>[2x]MSEFNITETYLRFLEEDTEMTMPIAAIEALVTLLRIKTPETAAEMINTIKSSTEELIKSIPNSVSLRAGCDIFMRFVLRNLHLYGDWENCKQHLIENGQLFVSRAKKSRNKIAEIGVDFIADDDIILVHGYSRAVFSLLNHAANKFIRFRCVVTESRPSKQGNQLYTLLEQKGIPVTLIVDSAVGAVIDKVDKVFVGAEGVAESGGIINLVGTYSVGVLAHNARKPFYVVTESHKFVRMFPLSSDDLPMAGPPLDFTRRTDDLEDALRGPTIDYTAQEYITALITDLGVLTPSAVSEELIKMWYD;>[2x]MSESEAKSRSATPPSKAKQATPTTTAAANGEKKLTNKELKELKKQEKAAKRAAMKQANGISIEQQQQQAQMKKEKKQLQREQQQKREQKQKNANKKKQNERNVKKSTLFGHLETTEERRATILALTSAVSSPKTSRITAAGLMVPVVASALSGSNVLTASSLMPVGPNASSTVSASAPASTTTTLPASSAALSAGTSSASTNTPTAIQQEIASSNASDVAKTLASISLEAGEFNVIPGISSVIPTVLEQSFDNSSLISSVKELLLNKDLIHPSILLLTSHLAHYKIVGSIPRCIAMLEVFQIVIKDYQTPKGTTLSRNLTSYLSHQIDLLKKARPLSVTMGNAIRWLKQEISLIDPSTPDKAAKKDLCEKIGQFAKEKIELADQLIIDNASTQIEESTTIVTYGSSKVLTELLLHNAISLKKNIKVIVVDSRPLFEGRKMAETLRNAGVNVMYALITSLDTIFNMDVDYVFLGAHSILSNGFLYSRAGTAMLAMSAKRRNIPVLVCCESLKFSQRVQLDSVTFNELADPNDLVNIDYENPVERRGNKGALLNQFIKERKFEKKKLAMENKPKGNKIGGKKGSEGESKDASNEEDSNSKNILDGWQELPSLNIVNILYDLTPPEYIKKVITEFGALPPSSVPVILREYKGSA;>MSSQAFTSVHPNAATSDVNVTIDTFVAKLKRRQVQGSYAIALETLQLLMRFISAARWNHVNDLIEQIRDLGNSLEKAHPTAFSCGNVIRRILAVLRDEVEEDTMSTTVTSTSVAEPLISSMFNLLQKPEQPHQNRKNSSGSSSMKTKTDYRQVAIQGIKDLIDEIKNIDEGIQQIAIDLIHDHEILLTPTPDSKTVLKFLITARERSNRTFTVLVTEGFPNNTKNAHEFAKKLAQHNIETLVVPDSAVFALMSRVGKVIIGTKAVFVNGGTISSNSGVSSVCECAREFRTPVFAVAGLYKLSPLYPFDVEKFVEFGGSQRILPRMDPRKRLDTVNQITDYVPPENIDIYITNVGGFNPSFIYRIAWDNYKQIDVHLDKNKA[2x];>MAGKKGQKKSGLGNHGKNSDMDVEDRLQAVVLTDSYETRFMPLTAVKPRCLLPLANVPLIEYTLEFLAKAGVHEVFLICSSHANQINDYIENSKWNLPWSPFKITTIMSPEARCTGDVMRDLDNRGIITGDFILVSGDVLTNIDFSKMLEFHKKMHLQDKDHISTMCLSKASTYPKTRTIEPAAFVLDKSTSRCIYYQDLPLPSSREKTSIQIDPELLDNVDEFVIRNDLIDCRIDICTSHVPLIFQENFDYQSLRTDFVKGVISSDILGKHIYAYLTDEYAVRVESWQTYDTISQDFLGRWCYPLVLDSNIQDDQTYSYESRHIYKEKDVVLAQSCKIGKCTAIGSGTKIGEGTKIENSVIGRNCQIGENIRIKNSFIWDDCIIGNNSIIDHSLIASNATLGSNVRLNDGCIIGFNVKIDDNMDLDRNTKISASPLKNAGSRMYDNESNEQFDQDLDDQTLAVSIVGDKGVGYIYESEVSDDEDSSTEACKEINTLSNQLDELYLSDDSISSATKKTKKRRTMSVNSIYTDREEIDSEFEDEDFEKEGIATVERAMENNHDLDTALLELNTLRMSMNVTYHEVRIATITALLRRVYHFIATQTLGPKDAVVKVFNQWGLLFKRQAFDEEEYIDLMNIIMEKIVEQSFDKPDLILFSALVSLYDNDIIEEDVIYKWWDNVSTDPRYDEVKKLTVKWVEWLQNADEESSSEEE[2x];>[2x]MSIQAFVFCGKGSNLAPFTQPDFPFQTQNKDSTAATSGDKLNELVNSALDSTVINEFMQHSTRLPKALLPIGNRPMIEYVLDWCDQADFKEISVVAPVDEIELIESGLTSFLSLRKQQFELIYKALSNSNHSHHLQDPKKINFIPSKANSTGESLQKELLPRINGDFVILPCDFVTDIPPQVLVDQFRNRDDNNLAMTIYYKNSLDSSIDKKQQQKQKQQQFFTVYSENEDSERQPILLDVYSQRDVTKTKYLQIRSHLLWNYPNLTVSTKLLNSFIYFCSFELCQLLKLGPQSMSRQASFKDPFTGNQQQQNPPTTDDDEDRNHDDDDDYKPSATSIQPTYFKKKNDLILDPINCNKSLSKVFRDLSRRSWQHSKPREPIGIFILPNETLFIRANNLNAYMDANRFVLKIKSQTMFTKNIQIQSAAIGADAIVDPKCQISAHSNVKMSVLGTQANIGSRCRVAGSLLFPGVHLGDEVILENCIIGPMAKIGSKCKLSNCYIEGHYVVEPKNNFKGETLANVYLDEDEEDELIYDDSVIAGESEIAEETDSDDRSDEDSDDSEYTDEYEYEDDGLFER;>[2x]MSTSHCRFYENKYPEIDDIVMVNVQQIAEMGAYVKLLEYDNIEGMILLSELSRRRIRSIQKLIRVGKNDVAVVLRVDKEKGYIDLSKRRVSSEDIIKCEEKYQKSKTVHSILRYCAEKFQIPLEELYKTIAWPLSRKFGHAYEAFKLSIIDETVWEGIEPPSKDVLDELKNYISKRLTPQAVKIRADVEVSCFSYEGIDAIKDALKSAEDMSTEQMQVKVKLVAAPLYVLTTQALDKQKGIEQLESAIEKITEVITKYGGVCNITMPPKAVTATEDAELQALLESKELDNRSDSEDDEDESDDE;>MSSDLAAELGFDPALKKKKKTKKVIPDDFDAAVNGKENGSGDDLFAGLKKKKKKSKSVSADAEAEKEPTDDIAEALGELSLKKKKKKTKDSSVDAFEKELAKAGLDNVDAESKEGTPSANSSIQQEVGLPYSELLSRFFNILRTNNPELAGDRSGPKFRIPPPVCLRDGKKTIFSNIQDIAEKLHRSPEHLIQYLFAELGTSGSVDGQKRLVIKGKFQSKQMENVLRRYILEYVTCKTCKSINTELKREQSNRLFFMVCKSCGSTRSVSSIKTGFQATVGKRRRM[2x];>[2x]MSDLQDQEPSIIINGNLEPVGEPDIVEETEVVAQETQETQDADKPKKKVAFTGLEEDGETEEEKRKREFEEGGGLPEQPLNPDFSKLNPLSAEIINRQATINIGTIGHVAHGKSTVVRAISGVQTVRFKDELERNITIKLGYANAKIYKCQEPTCPEPDCYRSFKSDKEISPKCQRPGCPGRYKLVRHVSFVDCPGHDILMSTMLSGAAVMDAALLLIAGNESCPQPQTSEHLAAIEIMKLKHVIILQNKVDLMREESALEHQKSILKFIRGTIADGAPIVPISAQLKYNIDAVNEFIVKTIPVPPRDFMISPRLIVIRSFDVNKPGAEIEDLKGGVAGGSILNGVFKLGDEIEIRPGIVTKDDKGKIQCKPIFSNIVSLFAEQNDLKFAVPGGLIGVGTKVDPTLCRADRLVGQVVGAKGHLPNIYTDIEINYFLLRRLLGVKTDGQKQAKVRKLEPNEVLMVNIGSTATGARVVAVKADMARLQLTSPACTEINEKIALSRRIEKHWRLIGWATIKKGTTLEPIA

Eukaryotic protein synthesis typically begins with a specialised initiator methionyl transfer RNA (Met-tRNAi) that is delivered to ribosomes by the translation factor eIF2 as part of a larger preinitiation complex (PIC) with multiple other translation initiation factors. Only by re-engaging with GTP can eIF2 participate in further rounds of Met-tRNAi binding and protein synthesis initiation. This requires the action of eIF2B. eIF2B first removes eIF57 and then acts as a guanine nucleotide exchange factor (GEF) to activate eIF2 and facilitate Met-tRNAi interaction and rebinding of eIF53. Structural studies of eIF2B have shown that it is a decamer or a dimer of pentamers. eIF2B has a central hexameric core comprising an eIF2Bα homodimer and (βδ)2 heterotetramer that is linked to a pair of γε heterodimeric arms. Here we have used single-particle electron cryomicroscopy (cryoEM) to resolve the structures of eIF2αP/eIF2B and eIF2/eIF2B complexes from Saccharomyces cerevisiae to an average resolution of 3.9 and 4.6 Å, respectively.

Purified PKR kinase was used to stoichiometrically phosphorylate eIF2α in vitro. eIF2αP/eIF2B complexes were generated by mixing the purified proteins and fractionating them by size exclusion chromatography. The final model shows two eIF2αγ complexes with a minimal eIF2β NTD helix, each bound at one side of a central eIF2B decamer. The resolution varies from 3.5 Å at the core to 18 Å at the periphery. Each eIF2αP is inserted between one eIF2Bα and 2Bδ and also makes contact with the adjacent eIF2Bβ to anchor eIF2αP to eIF2B. In contrast, each eIF2γ makes looser or transient contact with one adjacent lateral eIF2Bγε arm (see below). eIF2γ is the GDP/GTP binding subunit and is orientated so that the nucleotide-binding surface faces inwards towards eIF2B. However, upon eIF2B binding there is a local change. eIF2α residues 58–64 form a clear two-turn α-helix that is not observed in structures lacking eIF2B. The regulatory phosphoserine (serine 52 in S. cerevisiae and Homo sapiens eIF2α) sits in a conserved loop within domain 1 (residues 48–57) that contributes to the interface with eIF2B and is well resolved. Ser52 itself does not contribute directly to the interface with eIF2B, and the phosphate remains surface exposed. The positively charged side chains R54 and R64 are angled towards Ser52(P) and likely help stabilise this conformation of this important loop of eIF2α. However, in eIF2Bα side chains of T41 and E44 contact eIF2α D84 and Y82, respectively (non-H atoms are within 4 Å).> SSLDDKPQFPGASAEFIDKLEFIQPNVISGIPIYRVMDRQGQIINPSEDPHLPKEKVLKLYKSMTLLNTMDRILYESQRQGRISFYMTNYGEEGTHVGSAAALDNTDLVFGQYREAGVLMYRDYPLELFMAQCYGNISDLGKGRQMPVHYGCKERHFVTISSPLATQIPQAVGAAYAAKRANANRVVICYFGEGAASEGDAHAGFNFAATLECPIIFFCRNNGYAISTPTSEQYRGDGIAARGPGYGIMSIRVDGNDVFAVYNATKEARRRAVAENQ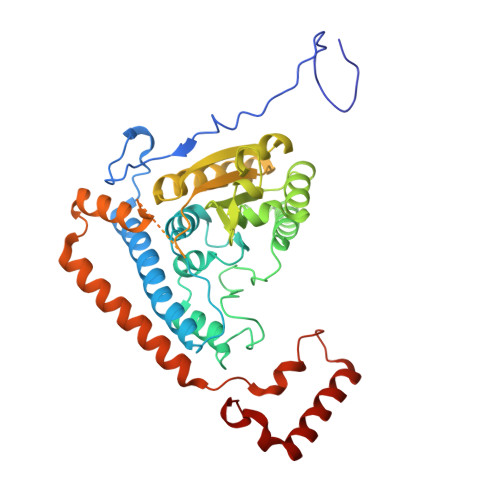PFLIEAMTYRIGHASTSADSSAFRSVDEVNYWDKQDHPISRLRHYLLSQGWWDEEQEKAWRKQSRRKVMEAFEQAERKPKPNPNLLFSDVYQEMPAQLRKQQESLARHLQTYGEHYPLDHFDK>[2x]MAKKTSS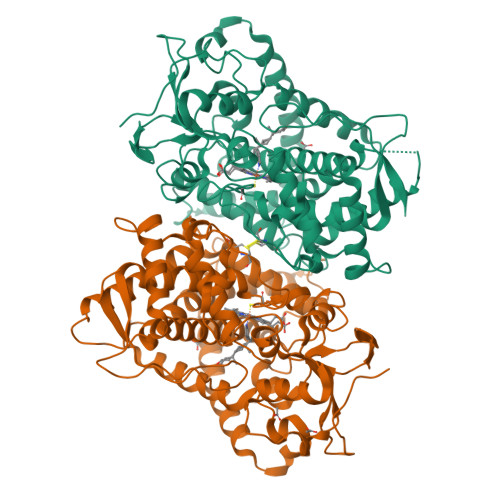KGKKQKMNGFVPAGNRSPPSLPSLPIIGSLMSLVSDSPPHIFFQDLQKKYGDLYSLMMGSHKLLIVNNHHHAKEILIKKGKIFAGRPRTVTTDLLTRDGKDIAFADYSSTWKFHRKMVHGALCMFGEGSVSIEKIICREASSMCEVLTESQNSAVDLGPELTRAVTNVVCALCFNSSYKRGDAEFESMLQYSQGIVDTVAKDSLVDIFPWLQIFPNKDLRILRQCISIRDKLLQKKYEEHKVTYSDNVQRDLLDALLRAKRSSENNNSSTRDVGLTEDHVLMTVGEIFGAGVETTTTTLKWSIAYLVHNPQVQRKIQEELDSKIGKERHPQLSDRGNLPYLEATICEVMRIRPVSPLLIPHVALQDSSVGEYTVQKGTRVVINMWSLHHDEKEWKNPELFDPGRFLNEEGDGLCCPSGSYLPFGAGVRVCLGEALAKMELFLFLAWILQRFTLEMPTGQPLPDLQGKFGVVLQPKKFKVVAKVRADWEKSPLMQHCHHHHHH>[6x]MRTLLIRYILWRNDNDQTYYNDDFKKLMLLDELVDDGDVSTLIKNMRMTLSDGPLLDRLNQPVNNIEDAKRMIAISAKVARDIGERSEIRWEESFTILFRMIETYFDDLMIDLYGEK

The VACV protein N1 was first described as a secreted protein but was shown subsequently to be a 14 kDa intracellular homodimer that is expressed early in the virus life cycle and contributes to virus virulence in mouse intradermal and intranasal models of infection. Functional analysis demonstrates that N1 inhibits apoptosis both in transfected cells and in VACV-infected cells and, consistent with this, biochemical analysis shows that N1 binds pro-apoptotic Bcl-2 family proteins Bad, Bax and Bid. The crystal structure of N1 reveals that it is a dimeric Bcl-2-like protein with a surface groove that is constitutively open and that is predicted by molecular modelling to bind BH3 motif peptides of pro-apoptotic Bcl-2 family members. N1 is the first VACV protein shown to be a Bcl-2 family member and represents another example of VACV anti-apoptotic proteins.

The full-length wild-type N1 and a C40S mutant were expressed in E. coli, purified, crystallized and the structure was solved at 2.9 Å resolution by MAD analysis of the selenomethionated protein. The C40S mutation was introduced to avoid intermolecular disulphide bond driven aggregation. The crystal contains three dimers per asymmetric unit. The structural model encompasses residues 1–114 (residues 115–7 were not visible in the electron density map) and has an Rfactor/Rfree of 23.7/24.4 %. Note that the C40S substitution is distal to the dimer interface. N1 contains seven α-helices arranged with a fold similar to Bcl-xL and other Bcl-2 family members, including viral counterparts. Comparison of N1 with Bcl-xL using program SHP matched 96 Cαs out of 114 with root-mean-square deviation (rmsd) 2.4 Å, and revealed secondary structure elements representing the BH motifs of Bcl-2 family members equivalent to those in Bcl-xL. The predominantly acidic surface of N1 contains a surface groove formed by helices α2, α3, α4 and the N terminus of α5. In contrast, the N1 groove has an open conformation that could readily bind BH3 regions of pro-apoptotic Bcl-2 proteins. The dimers of N1 observed in the crystal structure are held together by anti-parallel interactions between α1 and α6.>GPGGGGSGGGGSGELKAIAQELKAIAKELKAIAWELKAIAQGAGGSGSYFQSNAGGDQTEKTLKDIESAVIDMEVLSSTSVTQLVRDKQSARAYMAILDNEEEKARKLSVRNADPHVVSSTNALISRISMARAALAKAQAEMTSRMRPVVIMMCGPPGIGKTKAAEHLAKRLANEIRPGGKVGLVPREAVDHWDGYHGEEVMLWDDYGMTKIQEDCNKLQAIADSAPLTLNCDRIENKGMQFVSDAIVITTNAPGPAPVDFVNLGPVCRRVDFLVYCTAPEVEHTRKVSPGDTTALKDCFKPDFSHLKMELAPQGGFDNQGNTPFGKGVMKPTTINRLLIQAVALTMERQDEFQLQ[6x]

The viral non-structural protein NS3 is a membrane-bound AAA+ ATPase of superfamily 3 (SF3) with multiple proposed roles in the norovirus replication cycle. The full-length NS3 protein comprises a membrane-binding N-terminal domain (NTD), a helical bundle domain (HBD), and an AAA+ ATPase domain comprising Walker A, B, motif C, and arginine fingers (RR). SF3 helicases typically assemble into hexameric rings and couple ATP hydrolysis to conformational changes that generate mechanical force on nucleic acid substrates. Through integrative modeling, we propose that NS3 functions as a transmembrane RNA translocase, coupling membrane-associated genome replication to RNA transport.

In hex-NS3, the NTD (residues 1-61), is replaced by the 32-residue cc-hex coiled-coil sequence. The resulting structure shows that six copies of NS3 assemble into a funnel-shaped hexamer approximately 80 Å in height. The HBD and AAA+ ATPase domain form upper and lower tiers measuring ∼70 Å and ∼105 Å in diameter, respectively. Unlike the C6-symmetric model predicted by AlphaFold2, our cryo-EM reconstruction adopts a split lock-washer conformation, previously described in other AAA+ ATPases. The six subunits form a right-handed spiral with a rise of ∼1.5 Å per protomer and a gap of ∼6.5 Å between the topmost and bottommost subunits. Structurally, the HBD adopts a four-helix bundle (residues 64–148), connected to the AAA+ domain by a five-residue linker ([Fig fig2]). In our NS3 cryo-EM reconstruction, clear density corresponding to ATPγS is visible in all six nucleotide-binding sites, although it is less well resolved in protomer F, which lies at the seam of the hexamer ([Fig fig3]). In five of the six sites, resolved to ∼2 Å, we observed hexavalent coordination of a Mg²⁺ ion by the β- and γ-phosphates, the side chain of T169, and three water molecules. Subunits A–E show the γ-phosphate interacting with R276 and R277 (arginine finger), as well as with N259 (motif C), supporting their classification as ATP-bound. In contrast, subunit F adopts an apo-like conformation, as the arginine finger is displaced across the seam and does not engage the bound nucleotide ([Fig fig3]).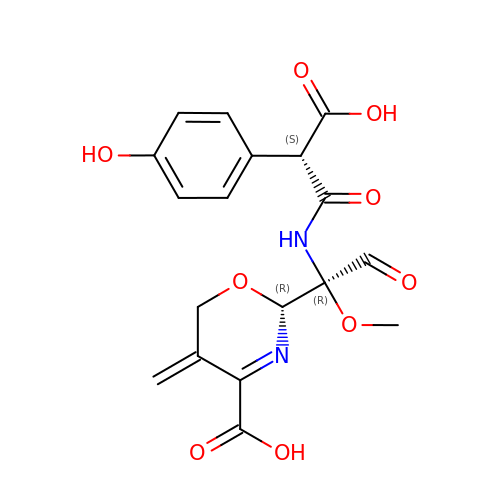(2R)-2-[(1R)-1-{[(2S)-2-carboxy-2-(4-hydroxyphenyl)acetyl]amino}-1-methoxy-2-oxoethyl]-5-methylidene-5,6-dihydro-2H-1,3-oxazine-4-carboxylic acid | C18 H18 N2 O9 | GOYCBKVVHGALFQ-RZAIGCCYSA-N>[4x]MHIQMTGQGVDISPALRELTEKKLHRIQPCRDEISNIHIIFHINKL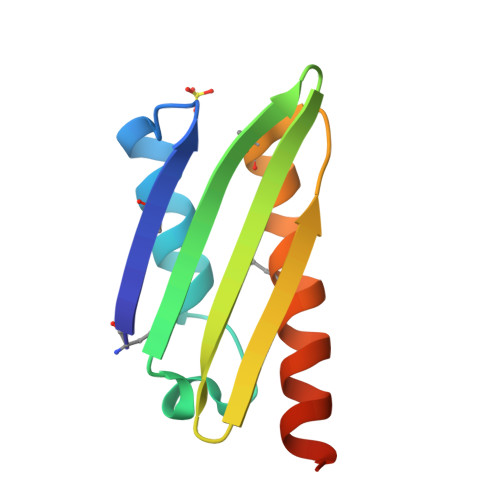KKIVDANVKLPGSTINAQAESDDMYKTVDLLMHKLETQLSKYKAKKGDHR Segmented negative strand RNA viruses of the arena-, bunya- and orthomyxovirus families uniquely carry out viral mRNA transcription by the cap-snatching mechanism. This involves cleavage of host mRNAs close to their capped 5′ end by an endonuclease (EN) domain located in the N-terminal region of the viral polymerase. The sNSV cap-snatching ENs belong to the PD-D/ExK superfamily of cation dependent nucleases. We find two different kinds of endonucleases, one with the characteristic catalytic histidine (His+) as in orthomyxovirus and bunyavirus, which have efficient endonuclease activity in isolation, and a second, without the histidine (His-) and conserved among arenaviruses which shows very poor activity in vitro.

Using a construct encompassing residues 1–174 from Lassa L protein we obtained three different crystal forms: one with no ions bound (crystal form X1), and two with one or two Mn2+ ions bound in the active site (crystal forms X2 and X3 respectively). The X2 data, solved by molecular replacement using the X1 structure, reached an ultra-high resolution of 1.09 Å, thus providing a highly accurate electron density map of the Lassa EN. In the X2 form, data measured close to the manganese absorption edge, showed a 50σ anomalous peak corresponding to one Mn2+ ion in the active. Compared with the X1 form, the X2 and X3 forms show a 17 degree rotation between the helical bundle lobe (residues 4–49 and 149–167) and residues 50–148, with the hinge being at the base of helix αb. The Lassa X2 structure has the same conformation as X3.

> GMEEDIACVKDLVSKYLADNERLSRQKLAFLVQTEPRMLLMEGLKLLSLCIEIDSCNANGCEHNSEDKSVERILHDHGILTPSLCFVVPDGYKLTGNVLILLECFVRSSPANFEQKYIEDFKKLEQLKEDLKTVNISLIPLIDGRTSFYNEQIPDWVNDKLRDTLFSLLRYAQES> MPRVKSYTGGTINFKEIESHLVGSSATARKDAVEALIAYFDGSRTQSQTTFDDKAYHRLFEALFRCTLIEKEAYFNSKKSVKVTAAAAARLERCPEALRLAVRHGVTTIRRKTARAIIDHIVQVLPGPDGAYVMPLLAGYVKVLYEFLDNPASAENIAALSGEGWEVCVDFCIDVLSRFLELGDRESGSLSRASPAPGATARSGSVAGTQGSGEQIGTHVAVDVLSCLYMLCIAHNAPIQRKADRLPHVVIQLLQLRQMKIGELQKMAFATFNIVFQRMQAEDVALCKTLVKQVVPLLSHWWQPRALSRDAMLNSIRDEMLKTLYGTRLYIQALLREAADESFPQDVEELLDTLWCDYSRREERARLQLDDITFTNMLLPPDHPRTGIFSLRPHHTAGEQNWALLENLAILEAAYSKHGQQEQSQQNQQQPEIDQPRKRRKMSGRQNRVHQKLHSLDPAVRLSALQLIPFLTRHKKPSLEDVAETLEDLSKHVTAKQAIVASWAMLACSSLAIHEVSRHPSLSSSWKQLWQLAVRSLSLPPISRASCVLLNSILKANLIPRHELADDINQIVTTADISGPAILVDASLGLMLNLLRFRNNMFPNASQATSNHIIRWVFVRWSPAELTYASLHGTHATPYDLVNLLRACYGISPLVMAQPLRLFNGPIVLHWKEQAEMEPFIRYLLLLHEEEPDTTVTPAQQEEQLPESNSATDVAGSNASRRLALELFYPKVEELQELAESWQKRGGEGATPVSMERLRSMVLACLTGALLLPDLVNINSSLSRDLESAVFSIVDATLKVILNSPPSENLFGMILASSAPYIPHLIEPELIALKRERPHLLKFFGKLSEALYERSRRESSHRDDQVIDIDPDFEPQTSQKNTASKAKTLPRRDILLSYTPEAFYLETSLRIHFLDIIRLNDGEIGRIPEPIINQLAGLSGEQFLCCREFMREIFTSDAIVPLGGATTILETAGHIVSRYEYACCEVALCNCIDIMDSFINLWTDNHFDIAEMAGDLYHYLVKQSLPNNSMSAAAQIRLASLLLHLLEVKSEYASNLGLPSSQSTLLKILQDGPMKLKHYIGLEIPKLFGLYVLKTHDDIFVDVLEHLPSDPDVVEGLAFRLFVLAELACRWPTLLRRSIYHTFEIPGKITKISKSQSCVTHSALYAASCIKRIAQTLKLSGPQELFKLFAPQLLYTWLDNDSIQDIAYEIFGFSSLLDLLREAQTEAAAIMMMRGQEQEVCQLAQSLGLTPEKLVQQSFTKIIAYSIAHDISIAGGPDYVTGESRMRKILGKEEYLANIHLNFADIISTFFDIFDQEDPIEKAFRRDERFAYAAETLEEIKKLGHLPTALPPNQQPMFRAKYLPREIVHLCSRTQYEPENIWTPALVVFVARKLLKTIHPALGPLHACSVLRKIRVLICLAGDHAISGYPLEMLLHSLRVFVVDPECADDALGITQYLIKRGDEYLKRTPSFLAGYALSSLADLRVFLSSSQSSTTQESQFKATKSKAQEFHAWFSKYLAAYDSPEFKDEGQKQAFRSITENAAHIRASGNAEKGTHESNLLLEILKDWGRENQLLNEPARDVALSMLCGVFNIPPSSRLDVIETDEDAIKNGAVVWKSCSSQRLGGEYLAWAGRVLGRSFAASGEVPEDLLRESQLQEYRRLSQGVGSSEEGLLNLIKSLTISGDCFTAGLAEAALRTIVSDAISDN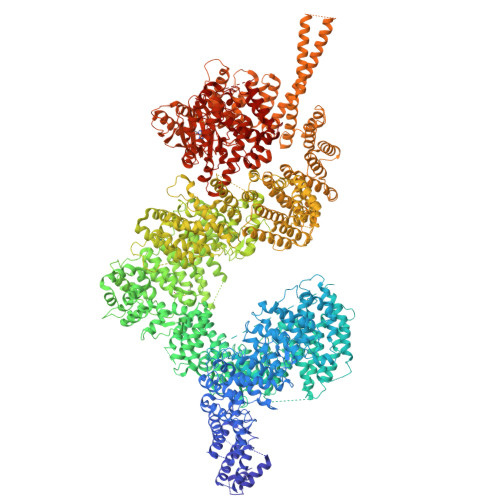DHDLLSACQESLPEPLLIASNWDPYRTPLSDQFKVDPPANTEVFSARALENPNWSQHLAIRLALSAPKIVTLRVLPPILSKVKGFAERAFPFVVHLVLAYQLDKQQSAKRELSESLQEWLNFTSEPAKENLKLLINTILYLRTQPLPGESSIADRAHWLDVNMASAAAAATRCGMYKVALLFAELAAESTRGSRRSSAARETDDSSDILLEIFENIDDPDAYYGLSQDASLSTVLARLEYENDGAKSLAFRGAQYDSHLRGRDLQSRQDCNALIKALSSLGLAGLSNSLLQSQQSIDGSSDSLDATFTTARKLEIWNLPAPVNSDSWAVTVYKAYQSMYQAQELDTVRSMVHDGLKNTVRHLSSGSLNTSVLRQQLGALAALTELDDILNVRDQSELQCTLATFEKRSKWMMSGRYADVSQILSCRETTLSMWSQRHNLRAAGLTSADARLVQIRGMLLSSDIFRFHRARQETLNLSTALSDLIPSCESLGLSVDAAIKMEAANALWDHGEMISSIRMLQAIDKDSSLKKQSVPLSRSDLLSKIGYQVSVARLESPDAIQKKYLEPALKELKGKIEGREAGQVFHQFAVFCDEQLQNPDSLEDLARLQNLKKGKDEEVAQLKALIASAKDSQLRNRYQSHLAKAKQWQELDQQELRRVEQTRSEFLKLCIENYLLSLAASDEHDNDALRFMALWLEKSEEEVANEVVKKWINKVPTRKFALLMNQLSSRLQDHNTLFQKLLIDLVYRICVDHPYHGMYHIWTGARTRVNKDDEVAVSRQRATDKIAKALSKNNKVSSIWPAIDQTSRVYHALAMDRDPTRYKSGQKVPIKNSPVGQNFLSTMSNNPIPPPTLQIEVSANLDYSHVPMIHKFAPEMAIASGVSAPKILTAIGTDGRKYKQLVKGGNDDLRQDAIMEQVFAAVSELLKLHRETRQRNLGIRTYKVLPLTSSSGLIEFVSNTIPLHEYLMPAHERYYPKDLKGSQCRKEIANAQTKNTETRIAVYRRVTERFHPVMRYFFMEYFPDPDEWFQKRTNYTRTTAAISMLGHVLGLGDRHGHNILLDHKTGEVVHIDLGVAFEMGRVLPVPELVPFRLTRDIVDGMGITKTEGVFRRCCEFTLDALREEAASIQTILDSLRHDTLYQWSISPVRMAKLQNAREVGGEDGGVGGGEDGEGGGVPKEKKQRPANEPSEADRAIEVVKKKLSKTLSVMATVNDLINQATSVSNLAVLYSGWAAYA> IVGGKVCPKGECPWQVLLLVNGAQLCGGTLINTIWVVSAAHCFDKIKNWRNLIAVLGEHDLSEHDGDEQSRRVAQVIIPSTYVPGTTNHDIALLRLHQPVVLTDHVVPLCLPERTFSERTLAF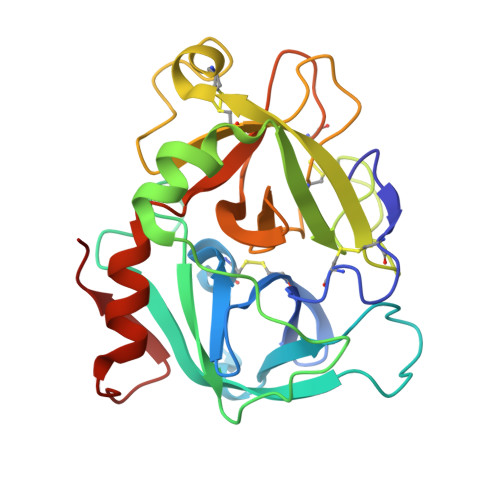VRFSLVSGWGQLLDRGATALELMVLNVPRVMTQDCEASYPGKITEYMFCAGYSDGSKDSCKGDSGGPHATHYRGTWYLTGIVSWGQGCATVGHFGVYTRVSQYIEWLQKLMRSEPRPGVLLRAPFP> MAFNPAPKAVQENHHVDYVIRFNYGDIDTPEAIKKFEVLLLELSEVGLQTEVRQGDENSLFVFVRAASKKKLKRAVYQSRVRDWLYGVRNTEPEPASSAKPQSEAERLLVIYHLITVPKAEGGAGITPRHGEWKNVDAIFPLHDEETNRQCMREWSKKTFLSTEDLDRIRNTFGEHVGFYFAFLQSYFRFLMFPAAFGFSCWLLLGSFSIIYTVVNCLWCIVFIEYWKRQEEDLSCRWQTKGVSAVHEKRAEFKPEKEIRDESTGEVRGVFPATKRMYRQLLQVPFALLAAVALGAIIATCFAIEIFISEVYNGPLKGYLVFIPTILVSALIPTMSAVLLTVATKLNDYENYETQDAYKVALTQKIFVVNFITSYLPIILTAFVYVPFASRIVPYLDVFHLTVRPFVSKEHAIKARTEFSINPDRLRKQVIYFTVTAQIVGFALETIVPFVKQ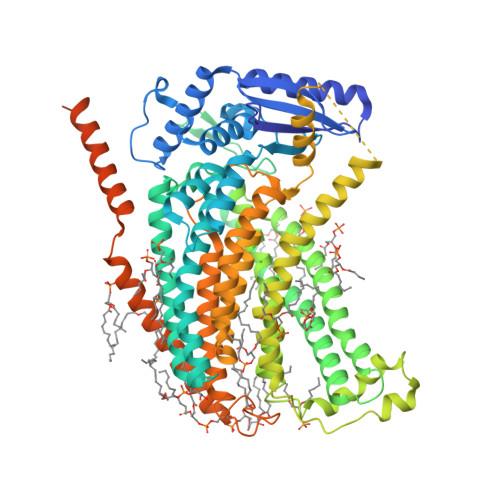RVFREYKEYTKKQHAKAEPGNGAGEKKTVSLGDDEDEARFLTRVRNEAELEDYDVTDDLREMCIQFGYLALFSPVWPLVPVSFLINNWVELRSDFFKICVECKRPWPQRADTIGPWLDSLGFLSWVGSITSSALVYMFSNGHEGPNGEPTTIRCWALLLTIFFSEHLYLIVRYAVRSALAKLEPPNTRRERIERFMMRKRYLDTVLSAESDDDADEVKGVVSSIPPSEITRESLEQDARDWSKQGTDPTERFWMRQRGWKESAEVGLSLITKAKGDETKKQQ> MAARLLAPPGPDSFKPFTPESLANIERRIAESKLKKPPKADGSHREDDEDSKPKPNSDLEAGKSLPFIYGDIPQGLVAVPLEDFDPYYLTQKTFVVLNRGKTLFRFSATPALYILSPFNLIRRIAIKILIHSVFSMIIMCTILTNCVFMTFSNPPDWSKNVEYTFTGIYTFESLVKIIARGFCIDGFTFLRDPWNWLDFSVIMMAYITEFVNLGNVSALRTFRVLRALKTISVIPGLKTIVGALIQSVKKLSDVMILTVFCLSVFALIGLQLFMGNLRNKCVVWPINFNESYLENGTKGFDWEEYINNKTNFYTVPGMLEPLLCGNSSDAGQCPEGYQCMKAGRNPNYGYTSFDTFSWAFLALFRLMTQDYWENLYQLTLRAAGKTYMIFFVLVIFVGSFYLVNLILAVVAMAYEEQNQATLEEAEQKEAEFKAMLEQLKKQQEEAQAAAMATSAGTVSEDAIEEEGEEGGGSPRSSSEISKLSSKSAKERRNRRKKRKQKELSEGEEKGDPEKVFKSESEDGMRRKAFRLPDNRIGRKFSIMNQSLLSIPGSPFLSRHNSKSSIFSFRGPGRFRDPGSENEFADDEHSTVEESEGRRDSLFIPIRARERRSSYSGYSGYSQGSRSSRIFPSLRRSVKRNSTVDCNGVVSLIGGPGSHIGGRLLPEATTEVEIKKKGPGSLLVSMDQLASYGRKDRINSIMSVVTNTLVEELEESQRKCPPCWYKFANTFLIWECHPYWIKLKEIVNLIVMDPFVDLAITICIVLNTLFMAMEHHPMTPQFEHVLAVGNLVFTGIFTAEMFLKLIAMDPYYYFQEGWNIFDGFIVSLSLMELSLADVEGLSVLRSFRLLRVFKLAKSWPTLNMLIKIIGNSVGALGNLTLVLAIIVFIFAVVGMQLFGKSYKECVCKINQDCELPRWHMHDFFHSFLIVFRVLCGEWIETMWDCMEVAGQAMCLIVFMMVMVIGNLVVLNLFLALLLSSFSADNLAATDDDGEMNNLQISVIRIKKGVAWTKLKVHAFMQAHFKQREADEVKPLDELYEKKANCIANHTGADIHRNGDFQKNGNGTTSGIGSSVEKYIIDEDHMSFINNPNLTVRVPIAVGESDFENLNTEDVSSESDPEGSKDKLDDTSSSEGSTIDIKPEVEEVPVEQPEEYLDPDACFTEGCVQRFKCCQVNIEEGLGKSWWILRKTCFLIVEHNWFETFIIFMILLSSGALAFEDIYIEQRKTI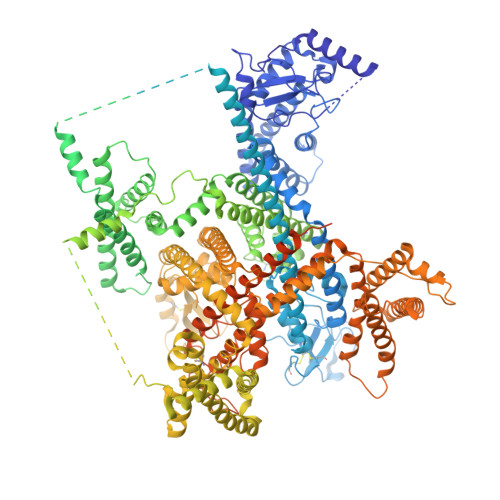RTILEYADKVFTYIFILEMLLKWTAYGFVKFFTNAWCWLDFLIVAVSLVSLIANALGYSELGAIKSLRTLRALRPLRALSRFEGMRVVVNALVGAIPSIMNVLLVCLIFWLIFSIMGVNLFAGKYHYCFNETSEIRFEIEDVNNKTECEKLMEGNNTEIRWKNVKINFDNVGAGYLALLQVATFKGWMDIMYAAVDSRKPDEQPKYEDNIYMYIYFVIFIIFGSFFTLNLFIGVIIDNFNQQKKKFGGQDIFMTEEQKKYYNAMKKLGSKKPQKPIPRPLNKIQGIVFDFVTQQAFDIVIMMLICLNMVTMMVETDTQSKQMENILYWINLVFVIFFTCECVLKMFALRHYYFTIGWNIFDFVVVILSIVGMFLADIIEKYFVSPTLFRVIRLARIGRILRLIKGAKGIRTLLFALMMSLPALFNIGLLLFLVMFIFSIFGMSNFAYVKHEAGIDDMFNFETFGNSMICLFQITTSAGWDGLLLPILNRPPDCSLDKEHPGSGFKGDCGNPSVGIFFFVSYIIISFLIVVNMYIAIILENFSVATEESADPLSEDDFETFYEIWEKFDPDATQFIEYCKLADFADALEHPLRVPKPNTIELIAMDLPMVSGDRIHCLDILFAFTKRVLGDSGELDILRQQMEERFVASNPSKVSYEPITTTLRRKQEEVSAVVLQRAYRGHLARRGFICKKTTSNKLENGGTHREKKESTPSTASLPSYDSVTKPEKEKQQRAEEGRRERAKRQKEVRESKC> MATVLIVGRPNVGKSTLFNKLVKKKKAIVEDEEGVTRDPVQDTVEWYGKTFKLVDTCGVFDNPQDIISQKMKEVTLNMIREADLVLFVVDGKRGITKEDESLADFLRKSTVDTILVANKAENLREFEREVKPELYSLGFGEPIPVSAEHNINLDTMLETIIKKLEEKGLDLESKPEITDAIKVAIVGRPNVGKSTLFNAILNKERALVSPIPGTTRDPVDDEVFIDGRKYVFVDTAGLRRKSRVEPRTVEKYSNYRVVDSIEKADVVVIVLDATQGITRQDQRMAGLMERRGRASVVVFNKWDLVVHREKRYDEFTKLFREKLYFIDYSPLIFTSADKGWNIDRMIDAMNLAYASYTTKVPSSAINSALQKVLAFTNLPRGLKIFFGVQVDIKPPTFLFFVNSIEKVKNPQKIFLRKLIR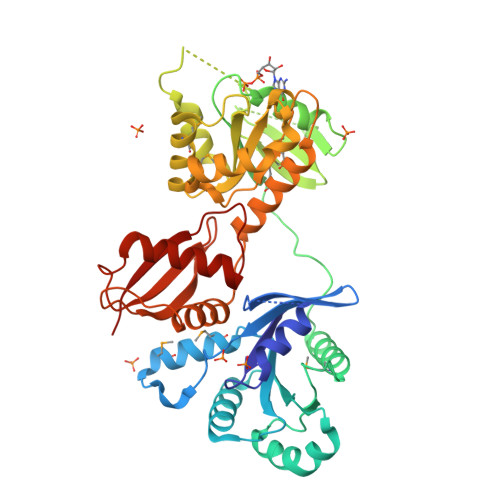DYVFPFEGSPIFLKFKRSR> PKQLRFEGERVTWIQASTLKELLDLKAQHPEAKLVVGNTEIGIEMKFKNQLFPMIICPAWIPELNAVEHGPEGISFGAACALSSVEKTLLEAVAKLPTQKTEVFRGVLEQLRWFAGKQVKSVASLGGNIITASPISDLNPVFMASGTKLTI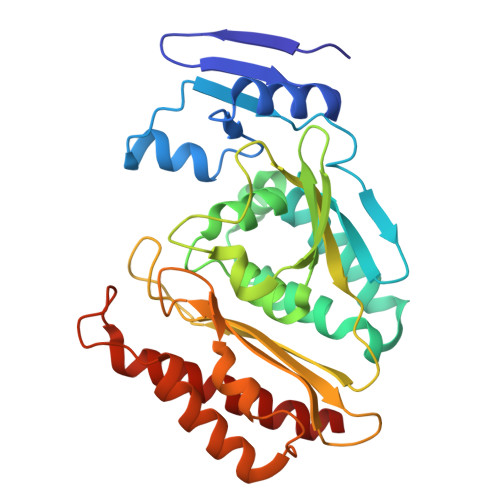VSRGTRRTVPMDHTFFPSYRKTLLGPEEILLSIEIPYSREDEFFSAFKQASRREDDIAKVTCGMRVLFQPGSMQVKELALCYGGMADRTISALKTTQKQLSKFWNEKLLQDVCAGLAEELSLSPDAPGGMIEFRRTLTLSFFFKFYLTVLKKLG>[2x]MTKPVLQDGETVVCQGTHAAIASE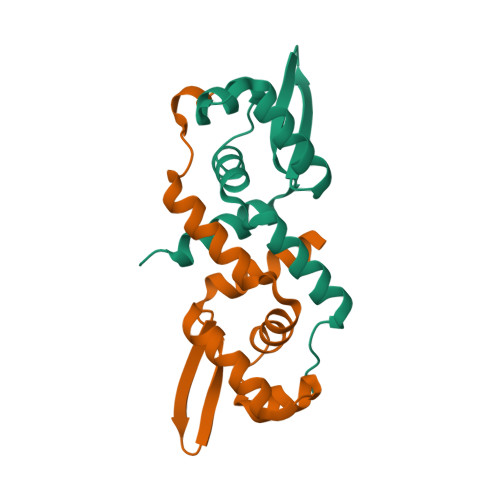LQAIAPEVAQSLAEFFAVLADPNRLRLLSLLARSELCVGDLAQAIGVSESAVSHQLRSLRNLRLVSYRKQGRHVYYQLQDHHIVALYQNALDHLQECR(1R,5S,6s)-3-[5-chloro-6-ethyl-2-(pyrimidin-5-yloxy)-7H-pyrrolo[2,3-d]pyrimidin-4-yl]-3-azabicyclo[3.1.0]hexan-6-amine | C17 H18 Cl 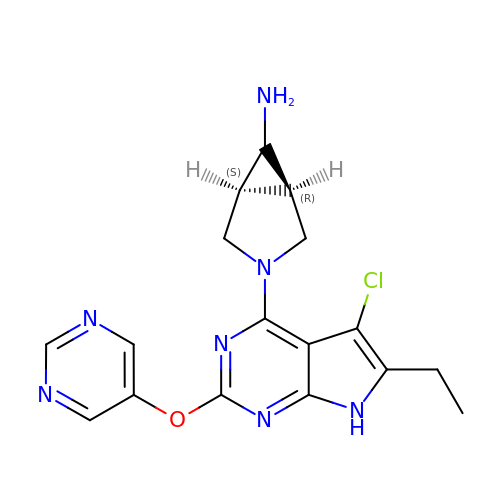N7 O | YZRGALHCPBRTES-MSRIBSCDSA-N> XYDYPGDHCY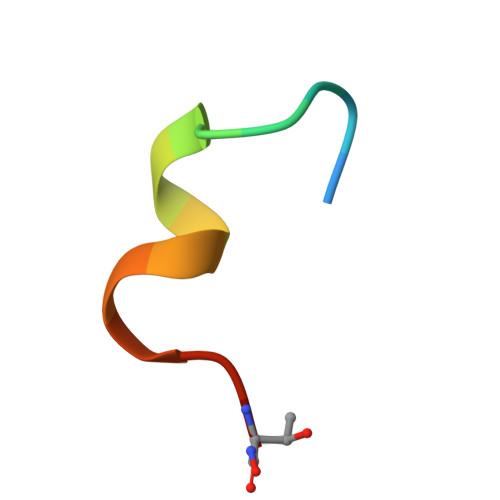LYGTX> MPSRTALSPGVLSPTRPVPNWIARPEYVGKPAAQEGSEPWVQTPEVIEKMRVAGRIAAGALAEAGKAVAPGVTTDELDRIAHEYLVDNGAYPSTLGYKGFPKSCCTSLNEVICHGIPDSTVITDGDIVNIDVTAYIGGVHGDTNATFPAGDVADEHRLLVDRTREATMRAINTVKPGRALSVIGRVIESYANRFGYNVVRDF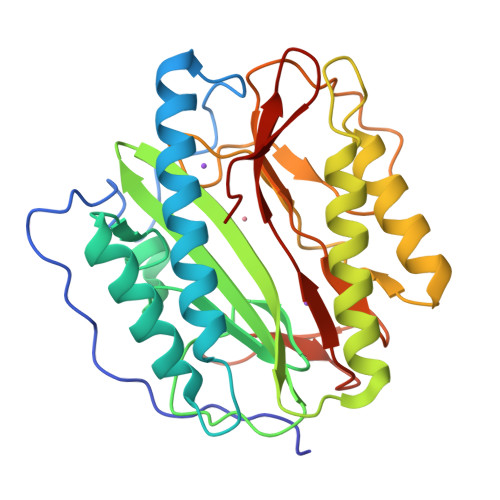TGHGIGTTFHNGLVVLHYDQPAVETIMQPGMTFTIEPMINLGALDYEIWDDGWTVVTKDRKWTAQFEHTLLVTDTGVEILTAL>AVKVGINGFGRIGRNVFRAALKNPDIEVVAVNDLTDANTLAHLLKYDSVHGRLDAEVSVNGNNLVVNGKEIIVKAERDPENLAWGEIGVDIVVESTGRFTKREDAAKHLEAGAKKVIISAPAKNEDITIVMGVNQDKYDPKAHHVISNASSTTNCLAPFAKVLHEQFGIVRGMMTTVHSYTNDQRILDLPHKDLRRARAAAESIIPTTTGAAKAVALVLPELKGKLNGMAMRVPTPNVSVVDLVAELEKEVTVEEVNAALKAAAEGELKGILAYSEEPLVSRDY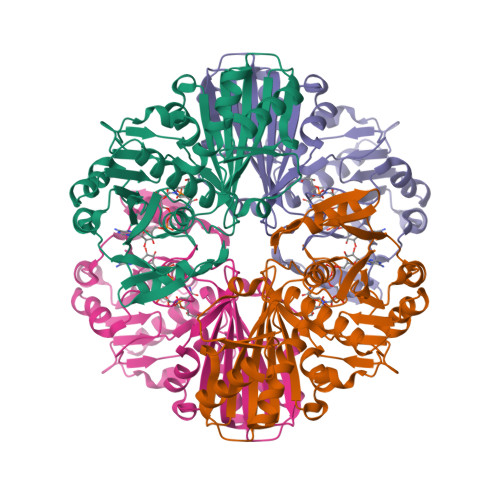NGSTVSSTIDALSTMVIDGKMVKVVSWYDNETGYSHRVVDLAAYIASKGL[4x]>[2x]MKSNSQNEKNGSETTNAVGNRKSVTVIGLGPMGQAMADVFLEYGYSVTVWNRTSSKADQLVAKGAIRVSTVNEALAANELVILSLTDYNVMYSILEPVSENLFGKVLV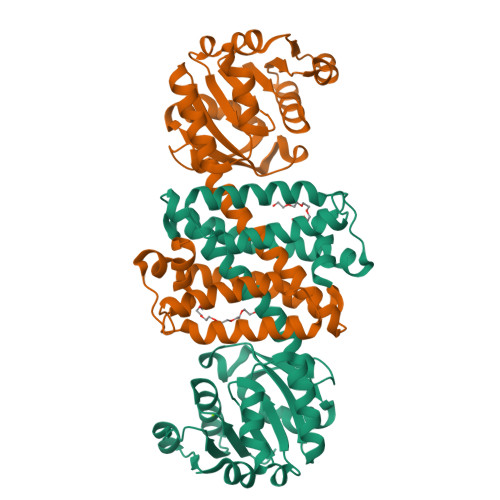NLSSDTPEKARKAAKWLEDRGARHITGGVQVPPSGIGKSESYTYYSGDRVVFEAHRETLEVLTSSDYRGEDPGLAMLYYQIQMDIFWTAMLSYLHALAIANANGITAEQFLPYASAMMSSLPKFVEFYTPRLDEGEHPGDVDRLAMGLASVEHVVHTTQEAGIDIALPATVLEVFRRGMKTGHASDSFTSLIEIFKNSDIRS> GSHMRLVSSEQALKELGLAEHQLRFTCRVHLHDTRKEQETALRVYS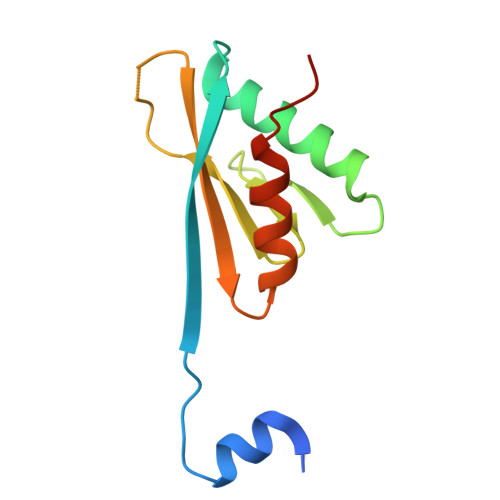HLKSVLKDHCVQHLPDGSVTVESVLLQAAAPSEDPGTKVLLVSWTYQDEELGSFLTSLLKKGLPQAPS methyl 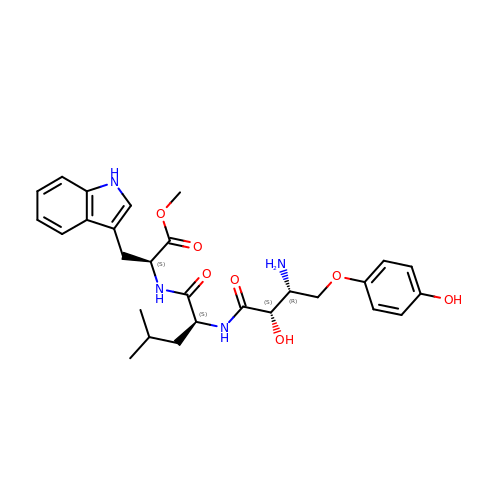(2S)-2-[[(2S)-2-[[(2S,3R)-3-azanyl-2-oxidanyl-4-(4-oxidanylphenoxy)butanoyl]amino]-4-methyl-pentanoyl]amino]-3-(1H-indol-3-yl)propanoate | C28 H36 N4 O7 | WXYVFLSKRTUFAE-VZVHPENPSA-N> MADSELQLVEQRIRSFPDFPTPGVVFRDISPVLKDPASFRAAIGLLARHLKATHGGRID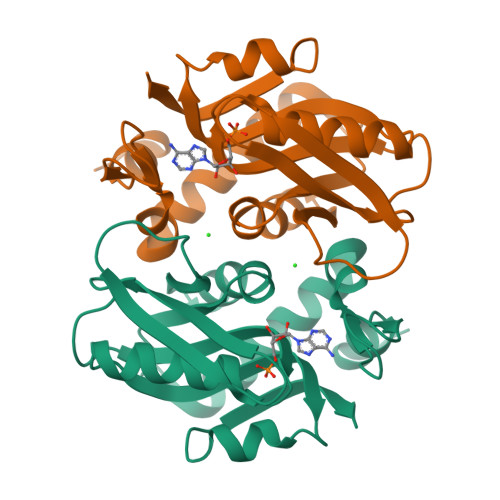YIAGLDSRGFLFGPSLAQELGLGCVLIRKRGKLPGPTLWASYSLEYGKAELEIQKDALEPGQRVVVVDDLLATGGTMNAACELLGRLQAEVLECVSLVELTSLKGREKLAPVPFFSLLQYE> QKPGETKEVHPQLTTFRCTKRGGCKPATNFIVLDSLWHWIHRAEGLGPGGCGDWGNPPPKDVCPDVESCAKNCIMEGIPDYSQYGVTTNGTSLRLQHILPDGRVPSPRVYLLDKTKRRYEMLHLTGFEFTFDVDATKLPCGMNSALYLSEMHPTGAKSKYNPGGAYYGTGYCDAQCFVTPFINGLGNIEGKGSCCNEMDIWEANSRASHVAPHTCNKKGLYLCEGEECAFEGVCDKNGCGWNNYRVNVTDYYGRGEEFKVNTLKPFTVVTQFLANRRGKLEKIHRFYVQDGKVIESFYTNKEGVPYTNMIDD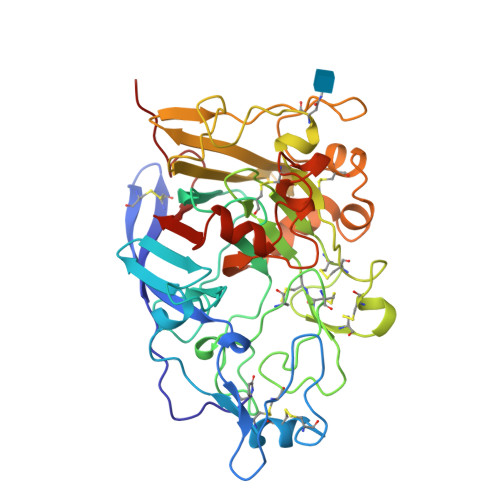EFCEATGSRKYMELGATQGMGEALTRGMVLAMSIWWDQGGNMEWLDHGEAGPCAKGEGAPSNIVQVEPFPEVTYTNLRWGEIGSTYQELQ> NLYQFKNMIQCTVPSRSWQDFADYGCYCGKGGSGTPVDDLDRCCQVHDNCYNEAENISGCRPYFKTYSYECTQGTLTCKGDNNACA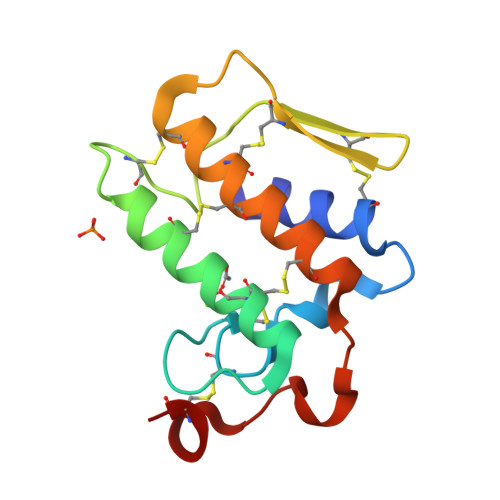ASVCDCDRLAAICFAGAPYNDANYNIDLKARCN> S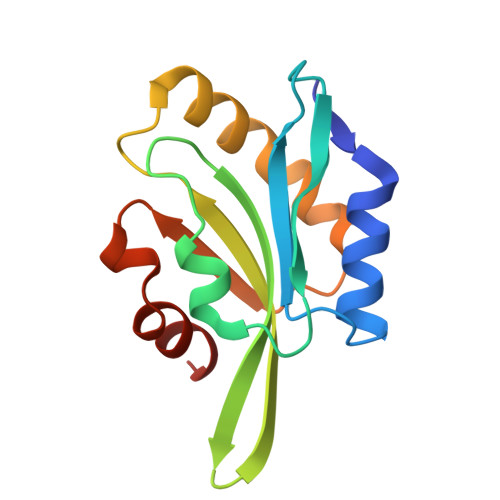GIAVSDDCVQKFNELKLGHQHRYVTFKMNASNTEVVVEHVGGPNATYEDFKSQLPERDCRYAIFDYEFQVDGGQRNKITFILWAPDSAPIKSKMMYTSTKDSIKKKLVGIQVEVQATDAAEISEDAVSERAKKDVK> MASVKLTELLDLYREDRGAKWVTALEEIPSLIIKGLSYLQLKNTKQDSLGQLVDWTMQALNLQVALRQPIALNVRQLKAGTKLVSSLAECGAQGVTGLLQAGVISGLFELLFADHVSSSLKLNAFKALDSVISMTEGMEAFLRGRQNEKSGYQKLLELILLDQTVRVVTAGSAILQKCHFYEVLSEIKRLGDHLAEKTSSLPNHSEPDHDTDAGLERTNPEYENEVEASMDMDLLESSNISEGEIERLINLLEEVFHLMETAPHTMIQQPVKSFPTMARITGPPERDDPYPVLFRYLHSHHFLELVTLLLSIPVTSAHPGVLQATKDVLKFLAQSQKGLLFFMSEYEATNLLIRALCHFYDQDEEEGLQSDGVIDDAFALWLQDSTQTLQCITELFSHFQRCTASEETDHSDLLGTLHNLYLITFNPVGRSAVGHVFSLEKNLQSLITLMEYYSKEALGDSKSKKSVAYNYACILILVVVQSSSDVQMLEQHAASLLKLCKADENNAKLQELGKWLEPLKNLRFEINCIPNLIEYVKQNIDNLMTPEGVGLTTALRVLCNVACPPPPVEGQQKDLKWNLAVIQLFSAEGMDTFIRVLQKLNSILTQPWRLHVNMGTTLHRVTTISMARCTLTLLKTMLTELLRGGSFEFKDMRVPSALVTLHMLLCSIPLSGRLDSDEQKIQNDIIDILLTFTQGVNEKLTISEETLANNTWSLMLKEVLSSILKVPEGFFSGLILLSELLPLPLPMQTTQVIEPHDISVALNTRKLWSMHLHVQAKLLQEIVRSFSGTTCQPIQHMLRRICVQLCDLASPTALLIMRTVLDLIVEDLQSTSEDKEKQYTSQTTRLLALLDALASHKACKLAILHLINGTIKGDERYAEIFQDLLALVRSPGDSVIRQQCVEYVTSILQSLCDQDIALILPSSSEGSISELEQLSNSLPNKELMTSICDCLLATLANSESSYNCLLTCVRTMMFLAEHDYGLFHLKSSLRKNSSALHSLLKRVVSTFSKDTGELASSFLEFMRQILNSDTIGCCGDDNGLMEVEGAHTSRTMSINAAELKQLLQSKEESPENLFLELEKLVLEHSKDDDNLDSLLDSVVGLKQMLES;>MHHHHHHHHHHSGDEVDAGSGHMTNEEPLPKKVRLSETDFKVMARDELILRWKQYEAYVQALEGKYTDLNSNDVTGLRESEEKLKQQQQESARRENILVMRLATKEQEMQECTTQIQYLKQVQQPSVAQLRSTMVDPAINLFFLKMKGELEQTKDKLEQAQN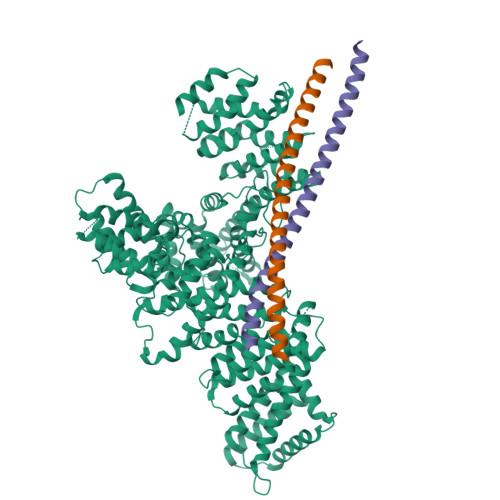ELSAWKFTPDSQTGKKLMAKCRMLIQENQELGRQLSQGRIAQLEAELALQKKYSEELKSSQDELNDFIIQLDEEVEGMQSTILVLQQQLKETRQQLAQYQQQQSQASAPSTSRTTASEPVEQSEATSKDCSRL[2x]> MTEETISQAVPPVRDWPAVDLPGSDFDPVLTELMREGPVTRISLPNGEGWAWLVTRHDDVRLVTNDPRFGREAVMDRQVTRLAPHFIPARGAVGFLDPPDHTRLRRSVAAAFTARGVERVRERSRGMLDELVDAMLRAGPPADLTEAVLSPFPIAVICELMGVPATDRHSMHTWTQLILSSSHGAEVSERAKNEMNAYFSDLIGLRSDSAGEDVTSLLGAAVGRDEITLSEAVGLAVLLQIGGEAVTNNSGQMFHLLLSRPELAERLRSEPEIRPRAIDELLRWIPHRNAVGLSRIALEDVEIKGVRIRAGDAVYVSYLAANRDPEVFPDPDRIDFERSPNPHVSFGFGPHYCPGGMLARLESELLVDAVLDRVPGLKLAVAPEDVPFKKGALIRGPEA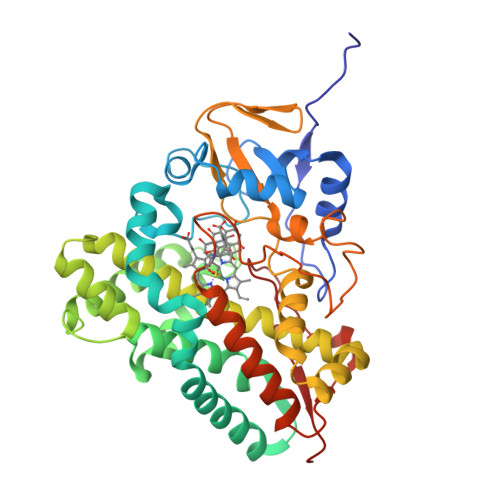LPVTWAAA>MGHHHHHHMVLMTKPGTSDFVWNGIPLSMELNLWNIKEYSGSVAMKFDGEKITFDADIQNLSPKEPERGGVLGYPEFYYGYKPWENHTAEGSKLPVPVSSMKSFSVEVSFDIHHEPSLPLNFAMETWLTREKYQTEASIGDVEIMVWFYFNNLTPGGEKIEEFTIPFVLNGESVEGTWELWLAEWGWDYLAFRLKDPVKKGRVKFDVRHFLDAAGKALSSSARVKDFEDLYFTVWEIGTEFGSPETKSAQFGWKFENFSIDLEVRE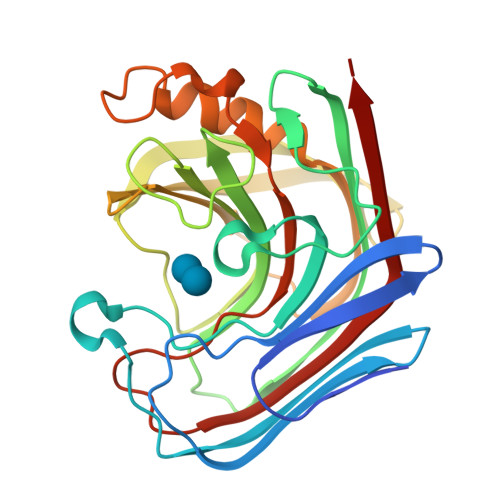[2x]> XCAIDQDFLDAAGILENEAIDIWNVTNGKRFSTYAIAAERGSRIISVNGAAAHCASVGDIV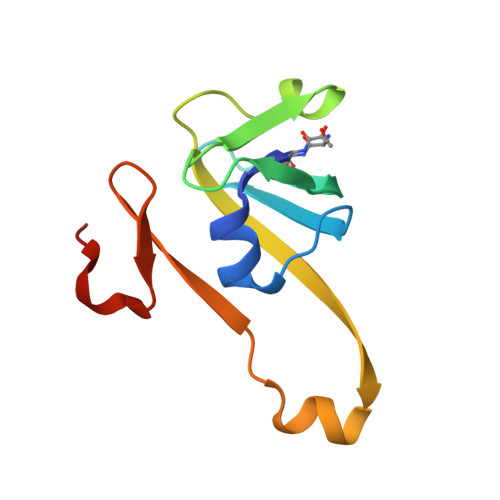IIASFVTMPDEEARTWRPNVAYFEGDNEMKRTAKAIPVQVA> ADLDNGEKVFSA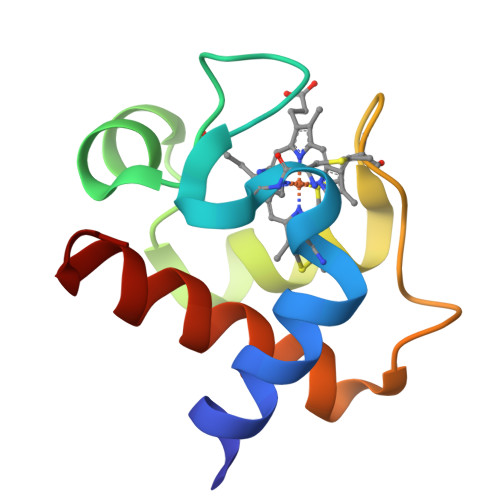NCAACHAGGNNAIMPDKTLKKDVLEANSMNTIDAITYQVQNGKNAMPAFGGRLVDEDIEDAANYVLSQSEKGW>SRCTHLENRDFVTGTQGTTRVTLVLELGGCVTITAEGKPSMDVWLDSIYQENPAKTREYCLHAKLSDTKVAARCPTMGPATLAEEHQSGTVCKRDQSDRGWGNHCGLFGKGSIVTCVKASCEAKKKATGHVYDANKIVYTVKVEPHTGDYVAANETHSGRKTASFTVSSEKTILTMGDYGDVSLLCRVASGVDLAQTVILELDKTSEHLPTAWQVHRDWFNDLALPWKHEGAQNWNNAERLVEFGAPHAVKMDVYNLGDHTGVLLKSLAGVPVAHIDGTKYHLKSGHVTCEVGLEKLKMKGLTYTMCDKTKFTWKRIPTDSGHDTVVMEVAFSGTKPCRIPVRAVAHGSPDVNVAMLITPNPIIENNGGGFIEMQLPPGDNIIYVGELSHQWFQKGSSIGRVFQKTRKGIERLTVIGEHAWDFGSAGGFLTSVGKALHTVLGGAFNSLFGGVGFLPKILVGVVLAWLGLNMRNPTMSMSFLLAGGLVLAMTL[3x];>VLIPSHAQGELTGRGHKWLEGDSLRTHLTRVEGWVWKNRLLALAMVTVVWLTLESVVTRVAVLVVLLCLAP[3x]

Tick-borne encephalitis virus (Orthoflavivirus encephalitidis, TBEV) is an enveloped single-stranded (+)RNA virus belonging to the Orthoflavivirus genus. Orthoflavivirus particles have icosahedral symmetry with a diameter of about 50 nm and a genome of about 11 kb. The glycoprotein shell of the mature infectious virion consists of 180 copies of each of membrane-anchored E (496 amino acid residues) and M proteins (75 amino acid residues). Envelope proteins E orchestrate the early stages of viral infection, virus entry into the cell and receptor-mediated endocytosis.

Formaldehyde-inactivated TBEV strain Sofjin-Chumakov is produced in the industrial scale for the vaccine manufacturing process and represents its antigen. In this study, we performed the first cryo-EM structure determination for the particles from the clinically approved TBE vaccine preparation based on a Far-Eastern subtype strain. It demonstrated the reliability of virus samples inactivated by cross-linking agents for structure determination and surface epitope analysis, which is especially important for emerging viruses. ELISA studies with monoclonal antibodies supported the hypothesis of TBEV protein shell cross-linking upon inactivation with formaldehyde.>[4x]MGHHHHHHMVPFCGHIKGGMRPGKKVLVMGIVDLNPESFAISLTCGDSEDPPADVAIELKAVFTDRQLLRNS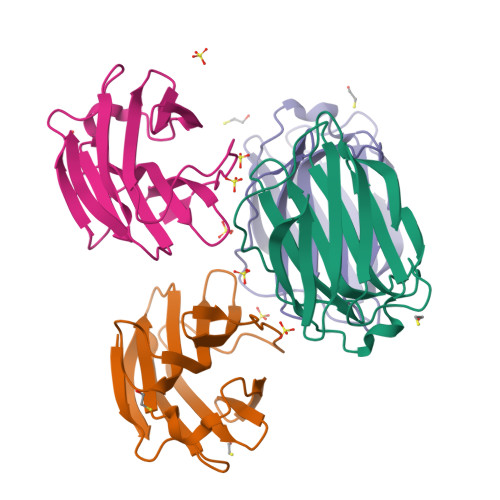CISGERGEEQSAIPYFPFIPDQPFRVEILCEYPRFRVFVDGHQLFDFYHRIQTLSAIDTIKINGDLQITKLG> HHHHHHMPSPNLPPGFDFTDPAIYAERLPVAEFAELRSAAPIWWNGQDPGKGGGFHDGGFWAITKLNDVKEISRHSDVFSSYENGVIPRFKNDIAREDIEVQRFVMLNMDAPHHTRLRKIISRGFTPRAVGRLHDELQERAQKIAAEAAAAGSGDFVEQVSCELPLQAIAGLLGVPQEDRGKLFHWSNEMTGNEDPEYAHIDPKASSAELIGYAMKMAEEKAKNPADDIVTQLIQADIDGEKLSDDEFGFFVVMLAVAGNETTRNSITQGMMAFAEHPDQWELYKKVRPE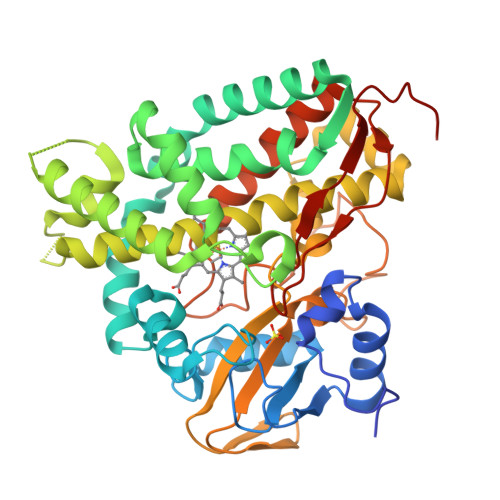TAADEIVRWATPVTAFQRTALRDYELSGVQIKKGQRVVMFYRSANFDEEVFQDPFTFNILRNPNPHVGFGGTGAHYCIGANLARMTINLIFNAVADHMPDLKPISAPERLRSGWLNGIKHWQVDYTGRLPVAH> MGHHHHHHMMRSHYCGQLNESLDGQEVTLCGWVHRRRDHGGVIFLDVRDREGLAQVVFDPDRAETFAKADRVRSEFVVKITGKVRLRPEGARNPNMASGSIEVLGYELEVLNQAETPPFPLDEYSDVGEETRLRYRFIDLRRPEMAAKLKLRARITSSIRRYLDDNGFLDVETPILGRPTPEGARDYLVPSRTYPGHFFALPQSPQLFKQLLMVAGFDRYYQIAKCFRDEDLRADRQPEFTQIDIETSFLDESDIIGITEKMVRQLFKEVLDVEFDEFPHMPFEEAMRRYGSDKPDLRIPLELVDVADQLKEVEFKVFSGPANDPKGRVAALRVPGAASMPRSQIDDYTKFVGIYGAKGLAYIKVNERAKGVEGLQSPIVKFIPEANLNVILDRVGAVDGDIVFFGADKAKIVCDALGALRIKVGHDLKLLTREWAPMWVVDFPMFEENDDGSLSALHHPFTSPKCTPAELEANPGAALSRAYDMVLNGT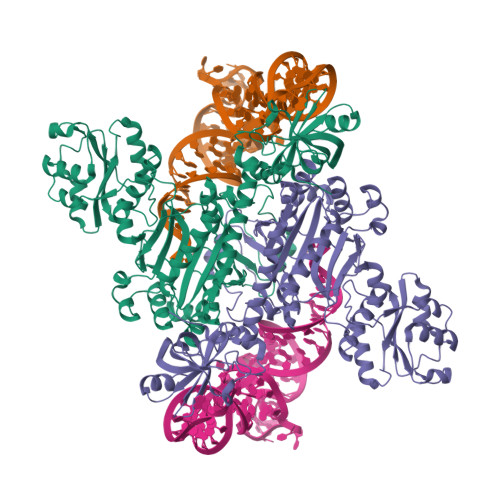ELGGGSIRIHDKSMQQAVFRVLGIDEAEQEEKFGFLLDALKYGAPPHGGLAFGLDRLVMLMTGASSIREVIAFPKTQSAGDVMTQAPGSVDGKALRELHIRLREQPKAE>[2x]KMPTLLRVYIDGPHGMGKTTTTQLLVALGSRDDIVYVPEPMTYWRVLGASETIANIYTTQHRLDQGEISAGDAAVVMTSAQITMGMPYAVTDAVLAPHIGGEAGSSHAPPPALTLIFDRHPIAALLCYPAARYLMGSMTPQAVLAFVALIPPTLPGTNIVLGALPEDR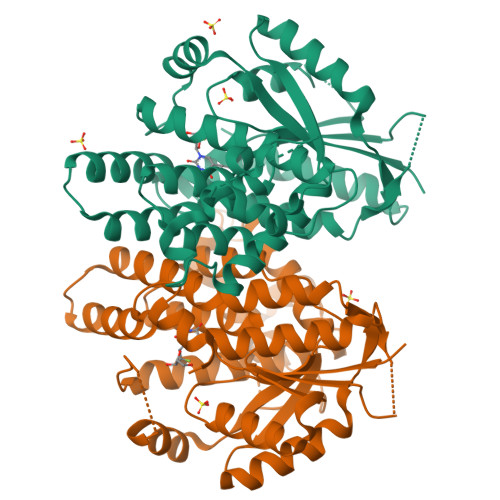HIDRLAKRQRPGERLDLAMLAAIRRVYGLLANTVRYLQCGGSWREDWGQLSGTAVPPQGAEPQSNAGPRPHIGDTLFTLFRAPELLAPNGDLYNVFAWALDVLAKRLRSMHVFILDYDQSPAGCRDALLQLTSGMVQTHVTTPGSIPTICDLARTFAREMGEAN> CCA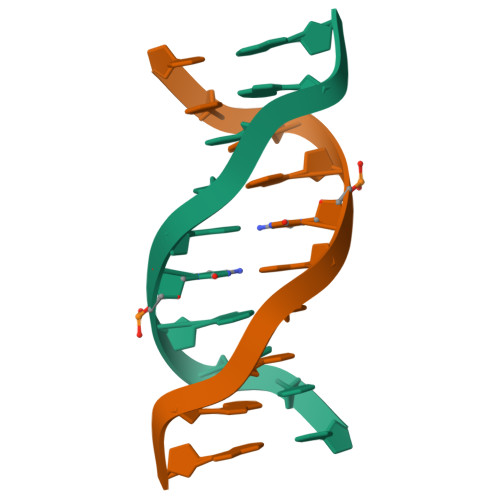GCGCTGG> MTNTLQVKLLSKNARMPERNHKTDAGYDIFSAETVVLEPQEKAVIKTDVAVSIPEGYVGLLTSRSGVSSKTHLVIETGKIDAGYHGNLGINIKNEHEDDKMQTIFLRNIDNEKIFEKERHLYKLGSYRIEKGERIAQLVIVPIWTPELKQVEEFESVSERGEK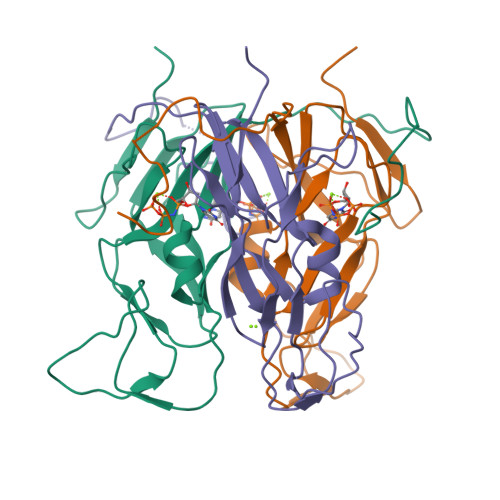GFGSSGV> GPGSMRPSLSDYQHVASGKVRELYRVDDEHLLFVATDRISAFDFVLDTPIPDKGRILTAMSVFFFGLLTVPNHLAGPPDDPRIPEEVLGRALLVRRLDMLPVECVARGYLTGSGLLDYQRTGAVCGHVLPQGLGEASRLDPPLFTPATKADIGEHDMNVDFAAVVGLVGAVRANQLRDETIKIYTRAAAHALHKGIILADTKF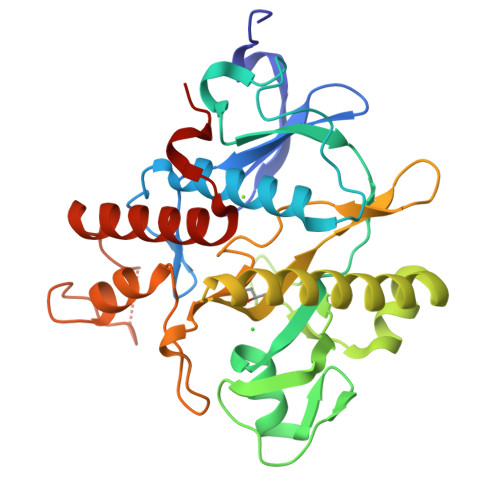EFGVDIEGNLVLADEVFTPDSSRYWDAAHYQPGVVQDSFDKQFVRNWLTGPESGWDRASDTPPPPLPDEVAVATRERYIEAYERISGLSFSDWIGPSA> HHHHHHAGQPEPVATPPAVDCATTKCVALTFDDGPGEYTNRLLDELSEQHTPATFFVLGKNVKKYPKTLKRMVDEGHQIGSHTFDHKDITKLTAEGIEHEVQWTDEAIEQAAGVKPQILRPPYGAHGAVYDRLIPYPLVLWDVDTLDWK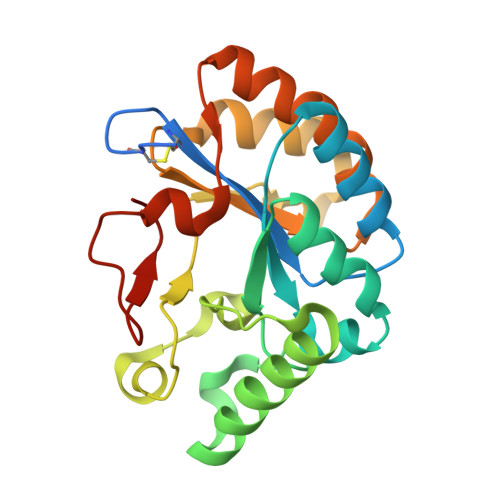HHDPQKTVRIALEEAKPGSIILMHDIHESSVKAVPQLVSKLHDAGYTLVTVDQLFAGTDFKPAKAYDHRFKTNP> QSLRSSLLGLRQLLRELPGDEAPLDALAETVLALLAQYGSLRIAGLYRVRYDRTPEPQPLATLGEMPALDADDLLVRTCLERGELVSVRQELLERGEQRAHSAAAVCVPLVDTDGRILALLAVEQMPFFVFNERTFSLLAILAGHIADLLQSD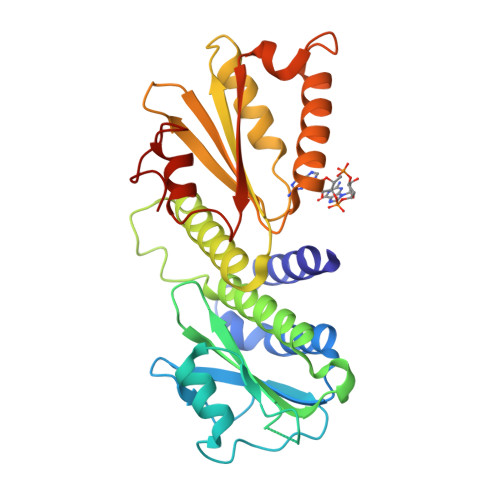RRALQLADIDAQRFSQYLKRSLLDARDHGLPACLYAFELTDARYGEEVQRLLEGSQRGLDVQLRLRNDEGRRVLLVLLPLTSAEGSQGYLQRLRILFAERFGQARELESLGVRIRQYELDAGNDRQALGHFLFNECGLNDQQVA>MTNPQFAGHPFGTTVTAETLRNTFAPLTQWEDKYRQLIMLGKQLPALPDELKAQAKEIAGCENRVWLGYTVAENGKMHFFGDSEGRIVRGLLAVLLTAVEGKTAAELQAQSPLALFDELGLRAQLSASRS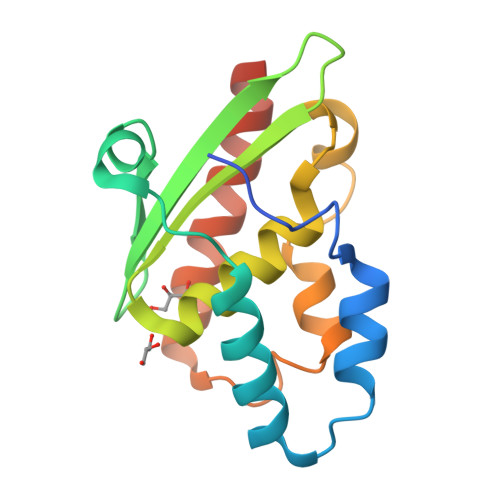QGLNALSEAIIAATKQVKHHHHHH[2x]> MHELIKYQFNTRRKKYGTGAALSLLNGNVGHEVLAFHKKLPNYAVTPLHNLAHLSQRLGLGSIHIKDESWRFGLNAFKGLGGSYAVGKYLADKLQCDINSLSFAALNTPEI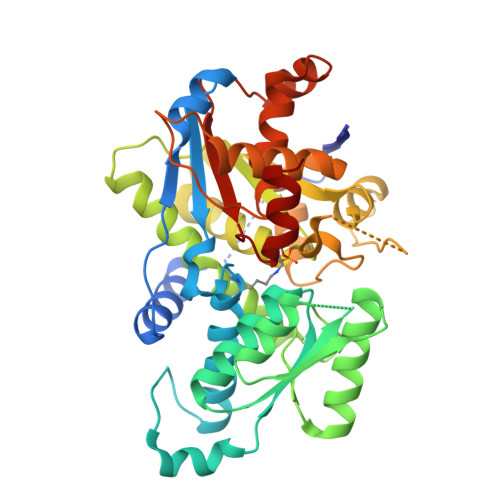KEKIKDCVFVTATDGNHGRGVAWAAEQLGLKAVVYMPKGSSLIRAENIRHHGAECTITDLNYDDAVRLAHRMAQTKGWVLLQDTAWTGYEEIPTWIMQGYMTLAVEAYEQLAETNSPLPTHLILQAGVGSFAGSVMGYFVEKMQENIPNIIVVEPHQANCLYQSAVMDDGQPHCVTGDMATIMAGLACGEPNIISWPIIRDNTSCFISADDCLAAKGMRISAAPRPGTDTPFISGESGAIGVGLLYELMNNMHYQDLANRLQLDASAHVLLISTEGDTSPDIYEDIVWNGRSA> EVKYPVVYEIFIRSLYDSDGDGVGDINGVSQKVDYLRKLGIDAVWFMPFNEAVSYHGYDITDYYNVEKDYGTMEDLENMIQVLHENGIKVIMDLVINHTSDEHPWFKDAVENTTSSPYWDYYIMSLEDHSGQDHWHWKINSKGQKVWYFGLFGYNMPDLNHDSQKVREEVKKIVDFWISKGVDGFRIDAAKHIYGWSWDDGIQESAEYFEWFRDYVLSKKPDAILVGEVFSGNTYDLSLYPIPVFNFALMYSIRNYPEGQDGMIENNWVEESFLFLENHDLHRFFSHLQEHYKKFSE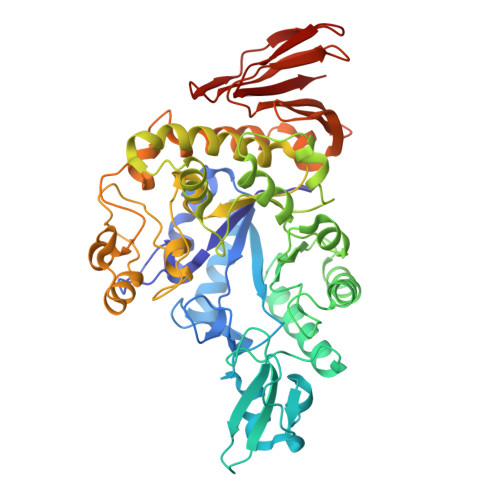SDYEFIKKRAALWYFLIFTLKGSPVIYYGGEIGTRGFKWHGPVYDEPVREPMQWYASGTGEGQTFWTKEVYKNAGITFGNADVDGCIYDDPYDGFSVEEQENDPKSLLNFIRFILNFRKDHDAILNGDQTIFRDWKNLIAFYRESSNEKLLVVLNPDPVWQNSFTFEENMTMILEVDFENFIWNESNVSFSAGESFTVDPMKAYIFKK> MNETPTRVYAEIDLDAVRANVRALRARAPRSALMAVVKSNAYGHGAVPCARAAQEAGAAWLGTATPEEALELRAAGIQGRIMCWLWTPGGPWREAIETDIDVSVSGMWALDEVRAAARAAGRTARIQLKADTGLGRNGCQPADWAELVGAAVAAQAEGTVQVTGVWSHFACADEPGHPSIRLQLDAFRDMLAYAEKEGVDPEV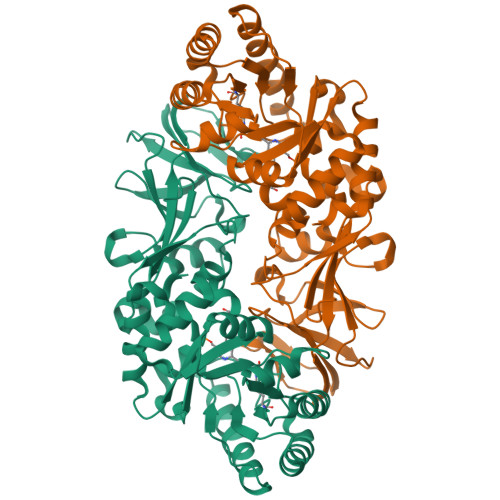RHIANSPATLTLPETHFDLVRTGLAVYGVSPSPELGTPAQLGLRPAMTLRASLALVKTVPAGHGVSYGHHYVTESETHLALVPAGYADGIPRNASGRGPVLVAGKIRRAAGRIAMDQFVVDLGEDLAEAGDEAVILGDAERGEPTAEDWAQAAHTIAYEIVTRIGGRVPRVYLGGLEHHHHHH> EACEMCR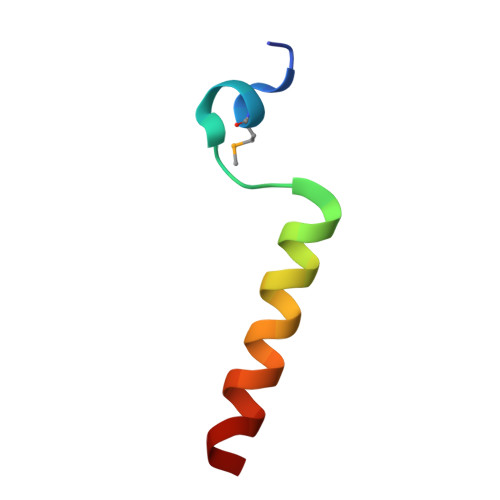LGLPHGSFFELLRDWKKIEEFRNKS>MKYQVKQVAEISGVSIRTLHHYDNIELLNPSALTDAGYRLYSDADLERLQQILFFKEIGFRLDEIKEMLDHPNFDRKAALQSQ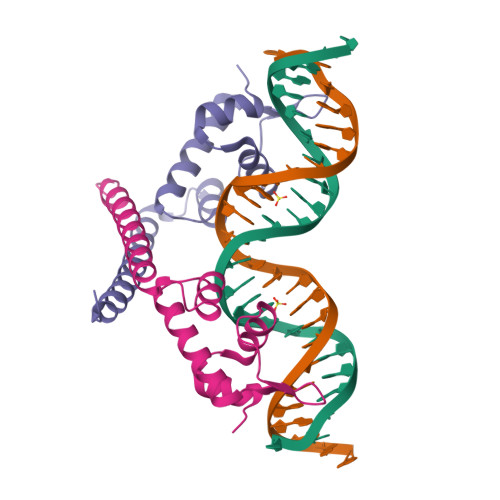KEILMKKKQRMDEMIQTIDRTLLSVD[2x]>MNSLLRLPALKRGVFTMSKRGLATTVSPKTRTSNLKNGLTIASESNPLVQTATVGVWIDAGSRNENAYNNGTAHFFEHLAFKGTDKRSQHQLELDIENMGGHLNAYTSRESTVYYAKSFKDDVPKSVEILADILQHSKLAESAIDREREVITRELEEVNKQYEEVVFDHLHATAFMNQPLGRTILGPRENIQTITNTELRKFITENYTADRMVLVGAGAVDHDALVELAEKYFSHLPSSQSPVPLGTPRSSGEDANQNPIPNFVGSEVRLRDDTMPVAHIAIAVEGVSWTSEDYYTALVAQAIIGNYDRAVGTSRHQGSRLSNIVSENNLANSFQSFSTSYSDTGLWGIYLTSENTTQIDDLVHFTLKEWNRLSTSVSNLQVERAKSQLKAGLLLSLDGTTYVAEDIGRQLTTLGRRVTPAEVEAKLEAVTEHDVRAWAQKTLYDKDIALVGLGPIEGLYDYNRIRNDMSMMRW[2x];>MTRGVPRLAVAARHFSTAEAAGVKVAAQDGQSPISDLSVVLRGGSRYATVPGVSHILEKFAFQNTVPKSALRFVRELELFGGKLYTHTTREHIVLRTQFLKQDLPYFVDAFANVLKETKFQQFELTERVAPVAELDLLKRESDPAFTALEAAHEVAFRTGLGNSVYAQGYSPVTLEDVKEFARQVYAKQNVAVVGNNVVPADLQQLVGTAFADLQEGSKVTQAGTTTLHGGEARVRTSTGNALTIALPIAEPKPVYHALASFLGGPASMPWSVGASPLAQATVGTHTSVKATYHNYGDAGLFAITIKGDSPAEISQVAHKAVQALKDTGAEVTEEQAARAYAKSKFAAAEAFENPDSSASVIGMELLSGVSRIAPENVQKFTPAELSEAAAQLSASAKPVVAAVGQVHALPFADELF[2x];>[2x]MALRKKNSLLNMANSYVLDSPQPSNLNYFWNFGSLLALCLVIQLATGITLAMHYTSHASLAFDSVEHIMRDVNFGWFIRYAHANTASFFFICIYAHMGRNIYYGSYKTPRVLPWSIGVIIFLLLIITAFMGYVLVFGQMSLWGATVICNLVSAIPWLGEDIVHFLWGGFSVGNPTLQRFFALHYLMPFVLAVFALLHLIALHTAGSSNPLGITSNVDKLSMHPYYSFKDLITVFAFLLMFTLFVFFSPDKLGHPDNYIPANPMVTPASIVPEWYLLPFYAILRAIPDKLGGVIAMVAAILILLILPIVDRSIIRGNAFKPISKLLFGFFICNFLLLGVLGQVHIEPPFIVLGQICTIFYFSYFLILLPMVSTIENIFFYIGSLRK;>MRRRRIGVWPENRRVSRLWVSLSPRSCVTCPVPTNQNPPINNHHTPILTQMFKAIPLRQALLGISSAVCAGATTTYYYTTKAEAMTAAEHGLHPAEYPWPQNGMLSTFDHASLRRGYQVYKEVCAACHSLDRIAWRNLVGVTHTTDEAKAFAEELEYDDEPDDEGNPRKRPGKLADYIPGPYPNEQAARAANQGALPPDLSLIAKARHGGADYIFALLTGYPDEPPAGVVLAPGMNYNPYFPGGGIGMARTLFDGVVEYEDGTPATTSQMAKDVAAFLTWAAEPEHDERKKLGLKAIIVISAMLGLSVYIKKFKWSPIKNRKFIYNPPKN[2x];>MSLLRTAAQAVKAPKAYTPLVAAKAFAQTRSVSSQPIGGKSTYKIPDFTPYLKKDRNTDANRLFSYFMIGSFGMLSAAGAKATVQDFLSNMSASADVLAMAKVEVKLGAIPLGKNVIIKWRGKPIFIRHRTSEEIEEANEVNVATLRDPQTDDERVQKPEWLVMIGVCTHLGCVPIGEAGDFGGWFCPCHGSHYDISGRIRRGPAPLNLEIPEYDFADAETLVIG[2x];>[2x]MSYFLTLASEVAESLLPTVAFASEEEKEQDEPVEVESDDDESEEKEDDDEEEDEDDDDDDDDDEVPDPAIALHEAAAEGPCHDFKHHFDECVERVTKAQEAEDYDHAEYKEDCVEEFFHLQHCINDNTADKLFRVLK;>[2x]MASITSVVKTSELILKSPLLSKIVVPLAKTYVKFSGYRQLGFKMNDLIIEETPNMQLALRRLPPTESYDRVYRLIRATQFSLSHKLATGNDITKPEEDDHYLIPYILDVEAEAFEKDALDNLEVVKRK;>MGGNGHYMGWWGHMGSPPQKGIAGYTISPFAARPFAGVVHAAIFNTFRRTKNQALFVILPVSFFYYVWTQASEKNEWLYTKAGRHELAKALAE[2x];>[2x]MAWATTFYNVFVKRNSAFVATILASAFVFDMTFETAIDNFWDRINAGKQWKDIRHKYIEAAGDDDEDDE;>[2x]MICGEGDYVKKPSYKIVPHFLGFNIPTVSKWIPIFGIWGAAAGIGALFLIEGVPRTRQDILSKIPIIGEHWIREIPASDNPF

The cytochrome bc 1 complex, also known as respiratory complex III (CIII), in the electron-transfer chain of the inner mitochondrial membrane is a homodimer (CIII2) of two biochemically identical protomers. CIII2 catalyses the transfer of electrons from the lipophilic two-electron donor ubiquinol (QH2) to the water-soluble, one-electron acceptor protein cytochrome c, contributing to an electrochemical proton gradient across the membrane. Electron transfer within the complex occurs through the prosthetic groups of the three catalytic core subunits: heme b L and heme b H of cytochrome b (cyt b), heme c 1 of cytochrome c 1 (cyt c 1) and the [2Fe–2S] cluster of the iron–sulfur protein (ISP), often called the Rieske protein after its discoverer. The Rieske domain is tethered to the complex by one transmembrane helix and a connecting flexible linker that acts as a hinge.

(v) +Atovaquone+antimycin A: with the Pf-type inhibitor atovaquone and the Qi-site inhibitor antimycin A. In crystallographic studies, problems of domain mobility can be overcome by Pf-type inhibitors, which fix the Rieske domain in the b position where its cluster-bearing tip is tightly docked to the surface of cyt b. The poor solubility of DQ limited the accessible concentration range, which may explain why we did not observe density in the Qi site in the consensus refinements. Atovaquone was resolved in the Qo site in the +atovaquone+antimycin A sample, with the Rieske domain fixed in the b position [Fig. 1(d)]. Atovaquone induced very tight binding of the tip of the Rieske domain to cyt b. As expected for a Pf-type inhibitor, the hinge region that tethers the mobile Rieske domain to the transmembrane domain was in an extended conformation. Together with the widening of the docking crater, this allowed close association of the Rieske domain with cyt b. Atovaquone formed a hydrogen bond to the cluster-ligating His190 (2.8 Å). In addition, Cys189, His170 and Leu171 of the Rieske domain formed hydrogen bonds to Tyr279, Lys288 and Asn149 of cyt b, as previously observed. These inter­actions stabilized the whole Rieske domain, improving the local resolution. As expected, the Rieske domain was mobile and thus poorly resolved, except when the Pf-type inhibitor atovaquone was added to arrest the domain at the surface of cyt b.>[3x]XGELKAIAQELKAIAKELKAIAWEHKAIAQGAGX;>[3x]X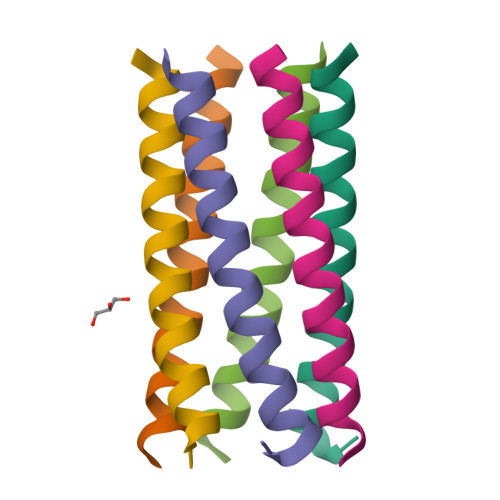GELKAIAQELKAIAYELKAIAKEDKAIAQGX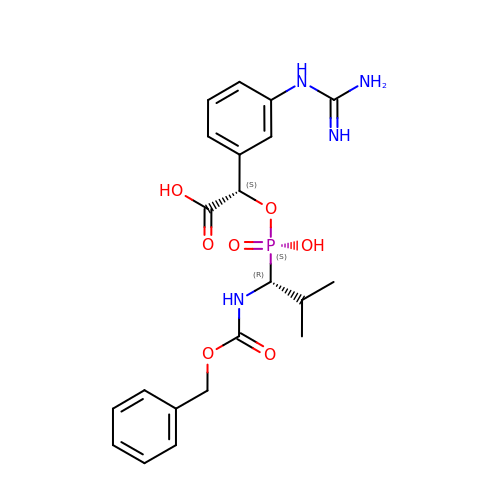(5R,6S,8S)-8-(3-{[AMINO(IMINO)METHYL]AMINO}PHENYL)-6-HYDROXY-5-ISOPROPYL-3-OXO-1-PHENYL-2,7-DIOXA-4-AZA-6-PHOSPHANONAN-9-OIC ACID 6-OXIDE | C21 H27 N4 O7 P | MGJJGNQEZQSCJT-ZWKOTPCHSA-N>[2x]DVQPETCRPSAASGNYFPQYPEYAIETARLRTFEAWPRNLKQKPHQ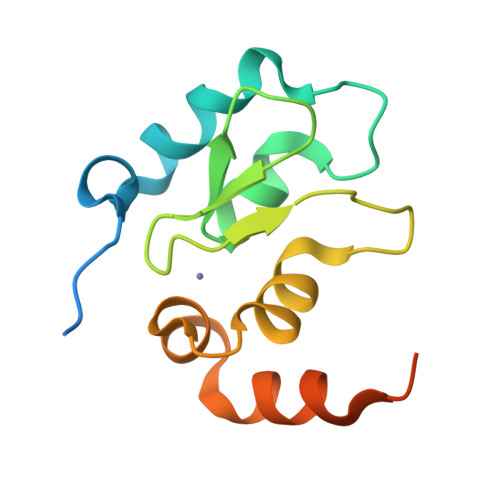LAEAGFFYTGVGDRVRCFSCGGGLMDWNDNDEPWEQHALWLSQCRFVKLMKGQLYIDTVAAKPVLAEEKEESTSIGGD> TIPHLAIDPFSLDFFDDPYPDQQTLRDAGPVVYLDKWNVYGVARYAEVHAVLNDPTTFCSSRGVGLSDFKKEKPWRPPSLILEADPPAHTRPRAVLSKVLSPATMKTIRDGFAAAADAKVDELLQRGCIDAIADLAEAYPLSVFPDAMGLKQEGREHLLPYAGLVFNAFGPPNELRQTAIERSAPHQAYVNEQCQRPNLAPGGFGACIHAFTDTGEITPDEAPLLVRSLLSAGLNTTVNGIGAAVYCLARFPGELQRLRSDPTLARNAFEEAVRFESPVQTFFRTTTREVELGGAVIGEGEKVLMFLGSANRDPRRWSDPDLYDITRKTSGHVGFGSGVHMCVGQLVARLEGEVMLSALARKVAAIDIDGPVKRRFNNTLRGLESLPV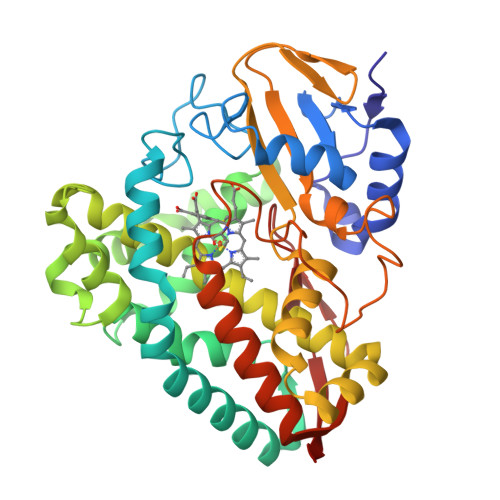KLTPA>GMEINADFTKPVVIDTDQLEWRPSPMKGVERRMLDRIGGEVARATSIVRYAPGSRFSAHTHDGGEEFIVLDGVFQDEHGDYPAGTYVRNPPTTSHVPGSAEGCTIFVKLWQFDPADRTQFSKNMEAELGA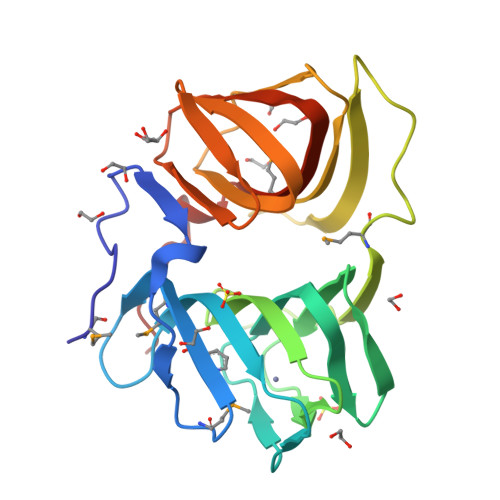PVEGISTSLLHEDERETVTHRKLEPGANLTSEAAGGIEVLVLDGDVTVNDEVLGRNAWLRLPEGEALSATAGARGAKIWMKTGHLRFVRTPEV[2x]> SGVDDDMACHKIPVEADFLYAYSTAP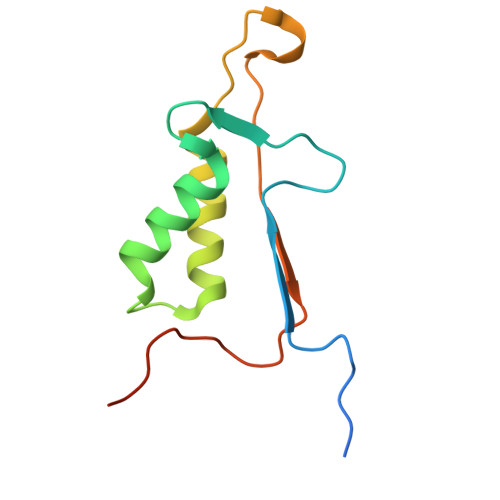GYYSWRNSKDGSWFIQSLCAMLKQYADKLEFMHILTRVNRKVATEFESFSFDATFHAKKQIPCIVSMLTKELYFYHLEHHHHHH The dot/icm T4bS system of L. pneumophila is powered by two ATPases: The membrane protein DotL, which is part of the coupling sub‐complex responsible for the recruitment of substrates and their delivery to the secretion channel and DotB, potentially involved in complex assembly and secretion. Here we present the X‐ray crystal structures of two DotB proteins, one from the dot/icm system encoded by the L. pneumophila genome (termed DotBL), at 3.19 Å resolution, and one from the dot/icm system encoded in the plasmid of Y. pseudotuberculosis IP31758 (termed DotBY), at 2.75 Å resolution. DotBL and DotBY subunits display a very similar topology. A DotBL or Y subunit is composed of a ∼150 aminoacids long N‐terminal domain (NTD), comprising 6 β‐strands and 3 α‐helices, and a ∼250 aminoacids C‐terminal domain (CTD) consisting of 7 β‐strands and 10 α‐helices [Fig. 1(A,B)]. The main part of the CTD adopts a RecA fold and harbours the signature motifs of the AAA+ family: The Walker A motif between β7 and α5 (also referred as P‐loop), the Asp Box on β8, the Walker B motif on β10 and the His Box on β11.

For the DotBL structure, two identical hexamers could be built, on top of each other, while only one is present in DotBY. The hinge point of this rotation is within the proline‐rich linker. In the hexamer, subunits A, C, and E adopt the α conformation, and subunits B, D, and F the β conformation, yielding an overall threefold symmetry [Fig. 2(C)]. DotBL was crystallized in the presence of AMP–PNP and ATPase activity assays using DotBL preincubated with increasing concentrations of AMP‐PNP show that the analogue binds and competes with ATP resulting in an inhibition of phosphate release. Yet, we could observe density for only phosphate not AMP–PNP. The phosphate is clamped by the main chain NH groups between residues 158 and 163 (TGSGKS) and by the Lys162 side chain. In the vicinity of this binding site (less than 6 Å away), the side chains of Glu191 (Asp box), Glu235 (Walker B) and His260 (His box), together with Arg221 (in α6) from the next subunit, point towards the ligand. In the α‐subunits, the binding site is highly similar, except for n + 1 Arg221, which is further from the binding site due to the alternate conformation of the n + 1 subunit [Fig. 4(D)]. Overall, we concluded that disruption of this interface by mutating those two arginines leads to disruption of the hexamer.

>MASWSHPQFEKIEGRSMDNINLMPDEPTRFTPVFMDRMLEHAESLNASDITIQTGEPIFAEVYGRLLKITNRRLSNTELGDLINSIYGPNATTQLLSGKDIDTHYEFRPNRGVRYRYRVNATACLVEGHDAIQITLRTIPTTPPKLSTMNLPDNIIEAIAPQEGIVFITGATGSGKSTLLASIIRELIETSDSNRKVLTYESPIEFVYDEIETISAVVSQSEIPRHLPNFADGVRNALRRKPRLIMVGECRDAETISAALEAALTGHPVYTTLHTSGVAETMRRLVTSFSGEERLGRTIDILETIRLCIWQKLVPTVDERRVALREYLVFDEEVRDILLEGDPNEVTSATRKLVRQKGQLMTWDAKMKFEQGIISERVYKLIIAGAKEYQQ[12x]>GHMNDLIDTTEMYLRTIYDLEEEGVVPLRARIAERLEQSGPTVSQTVARMERDGLLTVAEDRHLELTKAGRARAISVMRKHRLAERLLVDVIGLEWEQVHLEACRWEHVMSEAVERKLVKLLGNPTTSPYGNPIPGLDELGVGDSVEPVDTDLRRVDEVARSGGGR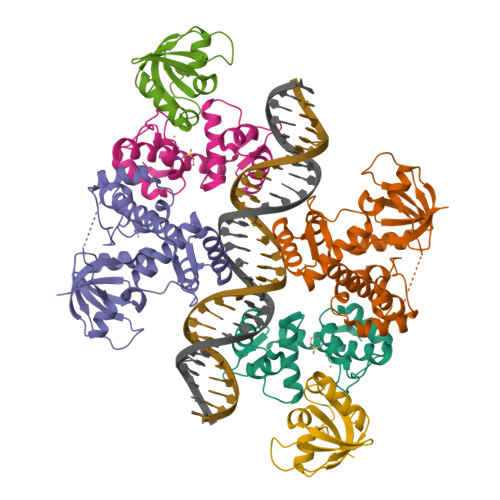ALVCRIAEHVQLDPDLMSELKKVGVVPGNEIDIVAVAGVNKPIQVQGSEGGTQLQPGIAHAVMVRVK[6x]> ECGHISVSAPIVHLGDPITASCIIKQNCSH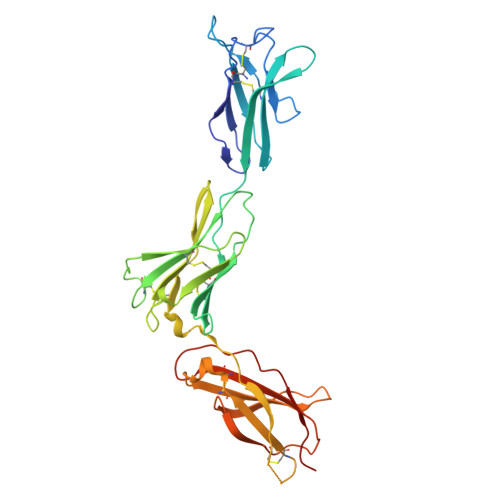LDPEPQILWRLGAELQPGGRQQRLSDGTQESIITLPHLNHTQAFLSCSLNWGNSLQILDQVELRAGYPPAIPHNLSCLMNLTTSSLICQWEPGPETHLPTSFTLKSFKSRGNCQTQGDSILDCVPKDGQSHCSIPRKHLLLYQNMGIWVQAENALGTSMSPQLCLDPMDVVKLEPPMLRTMDPSPEAAPPQAGCLQLSWEPWQPGLHINQKCELRHKPQRGEASWALVGPLPLEALQYELCGLLPATAYTLQIRCIRWPLPGHWSDWSPSLELRTTERAAAPR> MGNVQTSVNTYNITGDGNSFTPTSDMTSTAAPAIDLKPGVLNPTGKLWRPVGTSVATIDSLAIVSDRFGQYSFVNEGMRETFSKALFDINMWQPLFQATKTGCGPIVLSSFTTTTSGYVGATAGDALDNPVTNGVFISTVQIMNLQRTIAARMRDVALWQKHLDTAMTMLTPDISAGSASCNWKSLLAFAKDILPLDNLCLTYPNEFYNVAIHRYPALKPGNPDTKLPDAQAHPLGEVAGAFNAATSEVGSLVGSSSTLSQAISTMAGKDLDLIEADTPLPVSVFTPSLAPRSYRPAFIKPEDAKWIAEFNNSSLIRKTLTYSGATYTVQLGPGPTRVIDMNAMIDSVLTLDVSGTILPYDTNPDLSTSVPAFVLIQTSVPIQQVTTAANITAITVVSAAGAS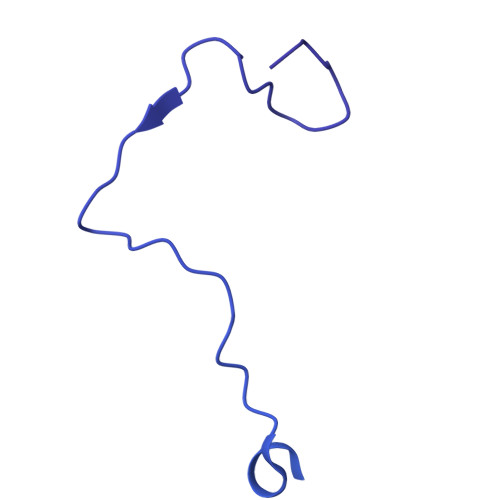AINLAINVRGQPRFNMLHLQATFERETITGIPYIYGLGTFLIPSPTSSSNFSNPTLMDGLLTVTPVLLRETTYKGEVVDAIVPATVMANQTSEEVASALANDAIVLVSNHLNKLANVVGDAIPVASRTDDSATSAIVSRLAVQHKLSQVGQASPTPPDYPLLWRRAKRAASMFVSNPSLALQVGIPVLTQSGMLSALTSGVGTALRTGSLGKGVTDASEKLRARQSLTVAKQAFFDQIGSLWPGK> RIIYDRKFLMECR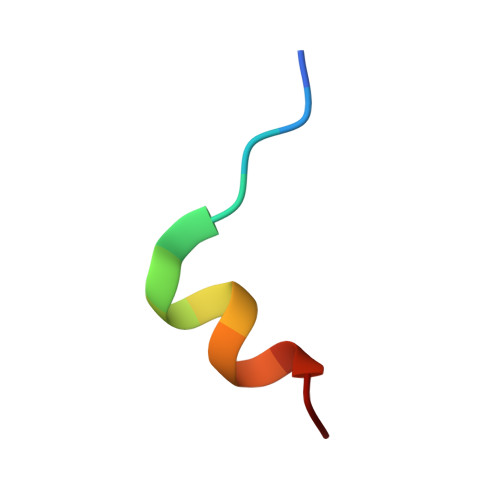N>NLPPGNYKKPKLLYCSNGGHFLRILPDGTVDGTRDRSDQHIQLQLSAESVGEVYIKSTETGQYLAMDTDGLLYGSQTPNEECLFLERLEENHYNTYISKKHAEKNWFVGLKKNGSCKRGPR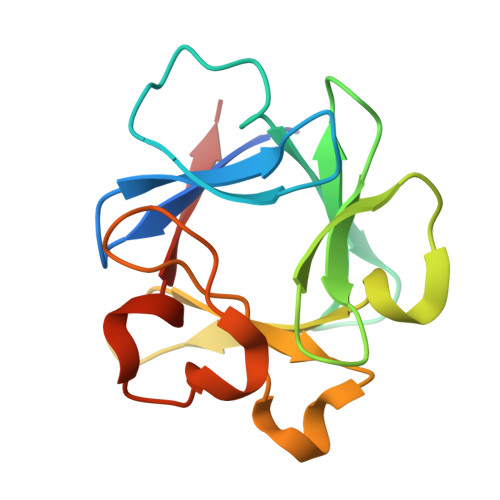THYGQKAILFLPLPVSSD[6x]>MGMKALILVGGFGTRLRPLTLSFPKPLVDFANKPMILHQIEALKAVGVDEVVLAINYQPEVMLNFLKDFETKLEIKITCSQETEPLGTAGPLALARDKLLDGSGEPFFVLNSDVISEYPLKEMLEFHKSHGGEASIMVTKVDEPSKYGVVVMEESTGRVEKFVEKPKLYVGNKINAGIYLLNPSVLDKIELRPTSIEKETFPKIAAAQGLYAMVLPGFWMDIGQPRDYITGLRLYLDSLRKKSPAKLTSGPHIVGNVLVDETATIGEGCLIGPDVAIGPGCIVESGVRLSRCTVMRG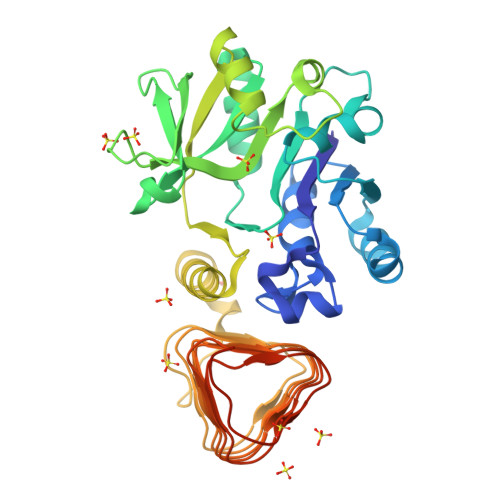VRIKKHACISSSIIGWHSTVGQWARIENMTILGEDVHVSDEIYSNGGVVLPHKEIKSNILKPEIVMKLAAALEHHHHHH[2x]>[12x]GSGSGSGMEKTQETVQRILLEPYKYLLQLP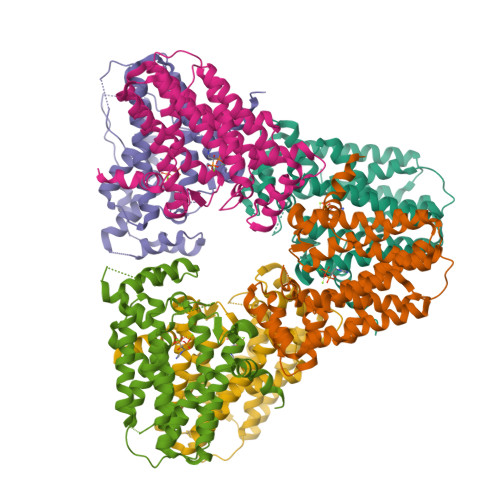GKQVRTKLSQAFNHWLKVPEDKLQIIIEVTEMLHNASLLIDDIEDNSKLRRGFPVAHSIYGIPSVINSANYVYFLGLEKVLTLDHQDAVKLFTRQLLELHQGQGLDIYWRDNYTCPTEEEYKAMVLQKTGGLFGLAVGLMQLFSDYKEDLKPLLNTLGLFFQIRYDYANLHSKEYSENKSFCEDLTEGKFSFPTIHAIWSRPESTQVQNILRQRTENIDIKKYCVHYLEDVGSFEYTRNTLKELEAKAYKQIDARGGNPELVALVKHLSKMFKEENE2,5 Furan Dicarboxylic Acid | C6 H4 O5 | 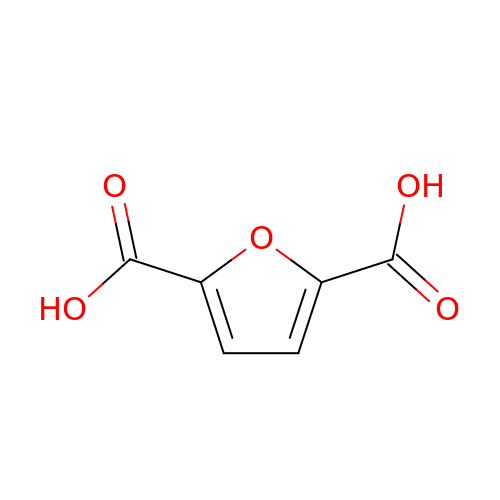CHTHALBTIRVDBM-UHFFFAOYSA-N> SASNYPAYMDNYLKEVINQVEEETGYNLLTTGMDVYTNVDQEAQKHLWDIYNTDEYVAYPDDELQVASTIVDVSNGKVIAQLGARHQSSNVSFGINQAVETNRDWGSTMKPITDYAPALEYGVYDSTATIVHDEPYNYPGTNTPVYNWDRGYFGNITLQYALQQSRNVPAVETLNKVGLNRAKTFLNGLGIDYPSIHYSNAISSNTTESDKKYGASSEKMAAAYAAFANGGTYYKPMYIHKVVFSDGSEKEFSNVGTRAMKETTAYMMTDMMKTVLSYGTGQNAYLAWLPQAGKTGTSNYTDEEIENHIKTSQFVAPDELFAGYTRKYSMAVWTGYSNRLTPLVGNGLTVAAKVYRSMMTYLSEGSNP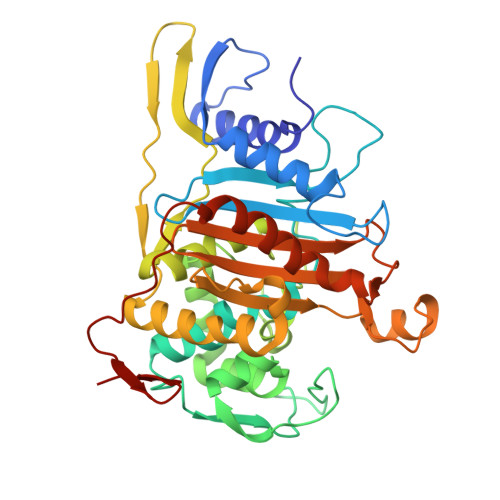EDWNIPEGLYRNGEFVFKNGAR(2R,3R,4S,5R,13R,14S,15R,16R)-24-amino-18-bromo-3,4,14,15-tetrahydroxy-7,9,11,25,26-pentaoxa-17,19,22-triaza-1-azonia-8,10-diphosphapentacyclo[18.3.1.1^2,5^.1^13,16^.0^17,21^]hexacosa-1(24),18,20,22-tetraene-8,10-diolate 8,10-dioxide 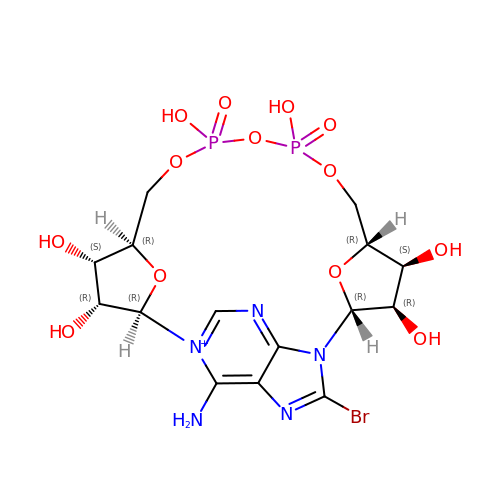| C15 H21 Br N5 O13 P2 | WDGMEOAIDHHBSJ-AIKIOGRUSA-M>[2x]SNANNARQARVAQSYENSYEVDSPAVRDSVLEAARQYNTSVVGFPILGPGLNRASKNSGPYLDYLQQLNPQR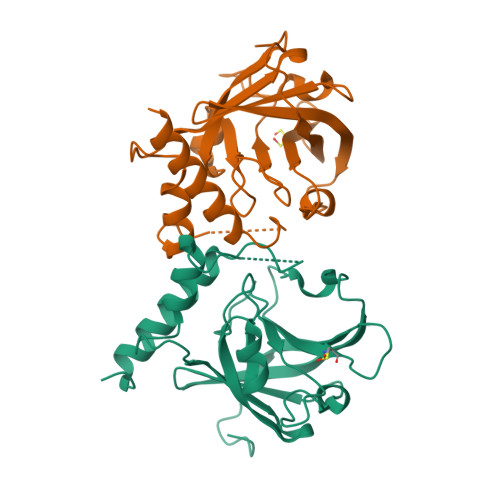AERPVIASISIPTIDAHLPIYHGTDTATLEHGLGHLYGSALPVGGTGTHPVITGHSGLANATLFDNLEDVKEHDPIYITVQGETLKYEVDAINVVLPEDTKLLAPDPNKDQITLITCTPYAVNSHRLLVRAHRVDLDPNDPNL>GSHMMKRLVYISKISGHLSLEEIQRIGKVSIKNNQRDNITGVLLYLQGLFFQILEGENEKVDKLYKKILVDDRHTNILCLKTEYDITDRMFPNWAMKTINLNENSELMIQPIKSLLQTITQSHRVLEKYMPARVIYLINQGINPLTVEPQLVEKIIFFSDILAFSTLTEKLPVNEVVILVNRYFSICTRIISAYGGEVTKFIGDCVMASFTKEQGDAAIRTSLDIISELKQLRHHVEATNPLHLLYTGIGLSYGHVIEGNMGSSLKMDHTLLGDAVNVAARLEALTRQLPYALAFTAGVKKCCQAQWTF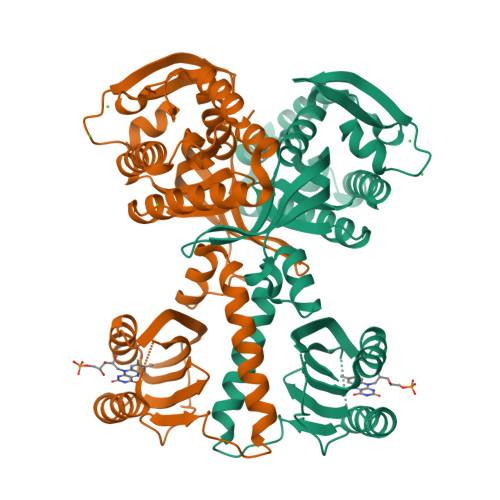INLGAHQVKGKQEAIEVYTVNEAQKYYDTLQITQLIRQTLENDK[2x]cyclopentyl {(2R,4S,6S,12Z,13aS,14aR,16aS)-2-[(7-methoxy-3-methylquinoxalin-2-yl)oxy]-14a-[(1-methylcyclopropane-1-sulfonyl)carbamoyl]-5,16-dioxo-1,2,3,5,6,7,8,9,10,11,13a,14,14a,15,16,16a-hexadecahydrocyclopropa[e]pyrrolo[1,2-a][1,4]diazacyclopentadecin-6-yl}carbamate 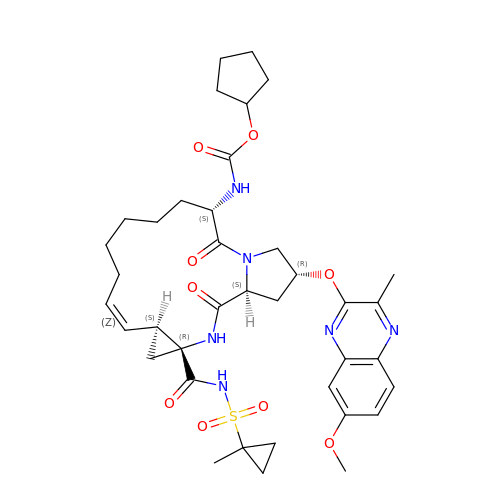| C38 H50 N6 O9 S | AWCLTDQQVULZEM-UIWVBJMMSA-N>GPKEWQENKSWNAHFTEHKSQGVVVLWNENKQQGFTNNLKRANQAFLPASTFKIPNSLIALDLGVVKDEHQVFKWDGQTRDIATWNRDHNLITAMKYSVVPVYQEFARQIGEARMSKMLHAFDYGNEDISGNVDSFWLDGGIRISATEQISFLRKLYHNKLHVSERSQRIVKQAMLTEANGDYIIRAKTGYSTRIEPKIGWWVGWVELDDNVWFFAMNMDMPTSDGLGLRQAITKEVLKQEKIIP[2x]

The OXA-48 carbapenemase is widely disseminated in Enterobacterales, necessitating new treatments for producer strains. OXA-48 is a class D SBL that uses a nucleophilic serine (Ser70) to hydrolyse β-lactams, with a proximal post-translationally carbamylated lysine (Lys73) proposed to act as the general base for both the acylation and deacylation steps of the reaction. Diazabicyclooctane (DBO) inhibitors, including avibactam and nacubactam, act on a wide range of enzymes to overcome β-lactamase-mediated resistance. Here we describe investigations on how avibactam and nacubactam inhibit OXA-48 and two variants, OXA-163 and OXA-405, with deletions in the β5–β6 loop neighbouring the active site that modify activity towards different β-lactam classes.

A crystal structure of nacubactam bound to homodimeric OXA-48 was solved at 1.51 Å resolution, from a crystal soaked with nacubactam for 30 min before freezing, with a chloride ion positioned at the dimer interface, as observed previously. Continuous positive Fo–Fc electron density between the ligand and Ser70 indicates the presence of a covalently bound nacubactam-derived carbamoyl-enzyme complex. The avibactam and nacubactam carbamoyl-enzyme complexes show a similar binding mode to OXA-48, with the nacubactam C7 carbonyl group positioned within the oxyanion hole formed by the backbone amides of residues Ser70 and Tyr211, as seen in β-lactam-derived acyl-enzyme complexes of OXA-48-like enzymes. In contrast, when Leu158 adopts the g-rotamer, observed when nacubactam is bound, the channel is closed, and the adjacent water is modelled in dual occupancy with the Leu158 side-chain, due we infer to steric clashes (Leu158 Cδ2 is ∼1.8 Å away from this water molecule). When OXA-48 is bound to nacubactam, in the active site of chain B, Arg214 of the Ω-loop adopts two conformations. In both conformations, the Arg214 side chain is poorly resolved in the final 2Fo–Fc electron density map. Thus, it is possible that the side chain of Arg214 and the C2 tail nitrogen of nacubactam are electrostatically repelled in crystallo due to clashing positive charges. Chain A of the nacubactam complex, in contrast, does not show this effect, most likely due to a crystal packing contact, whereby residue Glu132 from an adjacent molecule in a different asymmetric unit can electrostatically interact with Arg214, thus holding it in place. Consequently, the C2 tail group of nacubactam adopts a dual conformation in the chain A active site, presumably as a result of electrostatic repulsion by the Arg214 side chain. The structural studies reveal conformational variability of this loop only in the OXA-48 : nacubactam complex, as a result of electrostatic repulsion between the C2 tail nitrogen of the nacubactam 1-aminoethoxy group and the side chain of Arg214.(3-ENDO,8-ANTI)-8-BENZYL-3-(10,11-DIHYDRO-5H-DIBENZO[A,D][7]ANNULEN-5-YLOXY)-8-AZONIABICYCLO[3.2.1]OCTANE | C29 H32 N O | 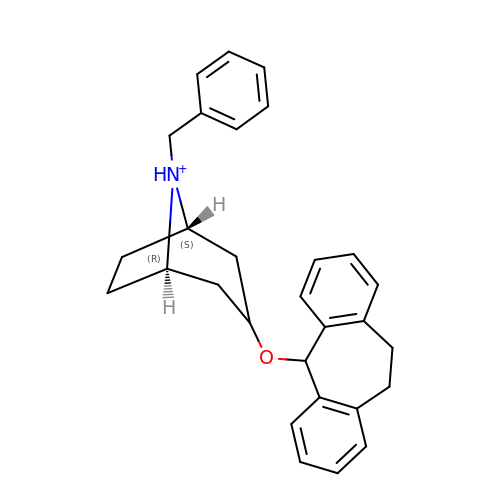DZOFIEFQFCWGIY-GPOLMCQNSA-O The solute carrier 13 (SLC13) family comprises electrogenic sodium ion–coupled anion cotransporters, segregating into sodium ion–sulfate cotransporters (NaSs) and sodium ion–di- and–tricarboxylate cotransporters (NaDCs). NaS1 and NaDC1 regulate sulfate homeostasis and oxidative metabolism, respectively. From an overall view, both the NaDC1 and NaS1 form a homodimer, and each protomer consists of 11 TMDs. The rest TMDs form the core domain that is responsible for substrate recognition and conformational change to complete the transport cycle.

For human NaS1, we captured both inward-facing conformations, namely, apo (NaS1_apo_IN/IN) and sulfate-bound states (NaS1_sulfate_IN/IN), achieving resolutions of 2.9 and 3.1 Å, respectively. The sulfate is coordinated by core domain of NaS1, which remains unchanged in different conformational states. In the structure of NaS1_IN/IN (top), sulfate stabilization relies on the side chains of Ser139 and Thr141 from HPin, as well as Thr259 and Ser260 of L5. Key residues participating in sulfate and sodium binding are from L5 and HPin of NaS1. A single sodium ion (named Na1) is distinctly coordinated within the NaS1 structure, involving the carbonyl oxygen atoms of Ser135 and Leu138, along with the side chain of Asn140 from HPin, and the carbonyl oxygen atoms of Gly258 on L5. The sodium density proposed to be bound around L10 and HPout is not found in cryo-EM map density. A notable variation is observed in Ser260 of NaS1, which is corresponding to the Pro201 in VcINDY, Gly288 in NaCT, and Ala241 in NaDC1 of L5, where Ser260 in NaS1 could potentially preclude citrate and succinate binding. (A) Cholesterol binding stabilizes the inward-open conformation of NaS1. During the transport cycle, the binding of cholesterol within NaS1-IN/IN induces the displacement of HPout in both horizontal and vertical directions with respect to the membrane plane.

>[2x]MADYKDDDDKSGRMKFFSYILVYRRFLFVVFTVLVLLPLPIVLHTKEAECAYTLFVVATFWLTEALPLSVTALLPSLMLPMFGIMPSKKVASAYFKDFHLLLIGVICLATSIEKWNLHKRIALKMVMMVGVNPAWLTLGFMSSTAFLSMWLSNTSTAAMVMPIAEAVVQQIINAEAEVEATQMTYFNGSTNHGLEIDESVNGHEINERKEKTKPVPGYNNDTGKISSKVELEKNSGMRTKYRTKKGHVTRKLTCLCIAYSSTIGGLTTITGTSTNLIFAEYFNTRYPDCRCLNFGSWFTFSFPAALIILLLSWIWLQWLFLGFNFKEMFKCGKTKTVQQKACAEVIKQEYQKLGPIRYQEIVTLVLFIIMALLWFSRDPGFVPGWSALFSEYPGFATDSTVALLIGLLFFLIPAKTLTKTTPTGEIVAFDYSPLITWKEFQSFMPWDIAILVGGGFALADGCEESGLSKWIGNKLSPLGSLPAWLIILISSLMVTSLTEVASNPATITLFLPILSPLAEAIHVNPLYILIPSTLCTSFAFLLPVANPPNAIVFSYGHLKVIDMVKAGLGVNIVGVAVVMLGICTWIVPMFDLYTYPSWAPAMSNETMP(3~{S},7~{R},10~{R},13~{S})-4-[[(3~{S},7~{R},10~{R},13~{S})-4-[(2~{S})-2-acetamido-3-(2-chlorophenyl)propanoyl]-2-oxidanylidene-1,4-diazatricyclo[8.3.0.0^{3,7}]tridec-8-en-13-yl]carbonyl]-2-oxidanylidene-1,4-diazatricyclo[8.3.0.0^{3,7}]tridec-8-ene-13-carboxylic 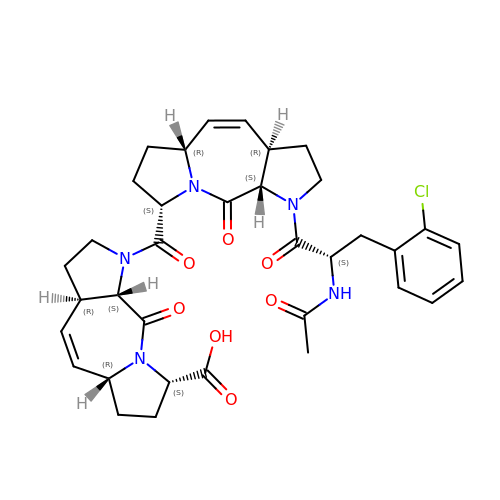acid | C35 H40 Cl N5 O7 | VTQUUKLGUPHTFW-DSSIVCCYSA-N Here we introduce Chroma, a generative model for proteins and protein complexes that can directly sample novel protein structures and sequences, and that can be conditioned to steer the generative process towards desired properties and functions. Given backbones from this diffusion process, the Chroma design network then generates sequence and side-chain conformations that are conditioned on the sampled backbone to yield a joint generative model for the sequences and structure of a protein complex. We sought to characterize the space of possible proteins parameterized by Chroma by generating a large number of unconditional samples of proteins and protein complexes (100,000 single-chain proteins and 20,000 complexes across two versions of the models, v.0 and v.1). The experimental characterization of 310 proteins shows that sampling from Chroma results in proteins that are highly expressed, fold and have favourable biophysical properties.

We reasoned that the best way to determine the plausibility of the protein space parameterized by Chroma was to draw independent samples from the model and test them experimentally. Our experimental validation shows that Chroma has learnt a sufficiently accurate distribution such that sampling from it results in proteins that express, fold, have favourable biophysical properties and conform to intended structures at non-trivial rates. The crystal structures of two designed proteins exhibit atomistic agreement with Chroma samples (a backbone root-mean-square deviation of around 1.0 Å). Moreover, the two designs with experimentally determined crystal structures demonstrate that a non-trivial fraction of this distribution should be expected to be atomistically accurate.

>MGSVEEVKRIMDLARQKISDAMDELNMDATLKQSVDESMKRAEQRAYELSKTHEKTDALGQASADLARELVARNTSEDHQKQIFEALKKAAEEMAHRSDSHEDRLVMALILQTYANAKVTFRILNSGKALGKEDEAQKMADRWTRLSAEAASLSVQAINDSTSAEKMAENFRQAKEDAVASLHRAGQDDLARKVSEFADAGLSKIDELMTLTGQMWAHGLFSKEWEDAARSLSRLAAVMLAQASQTKEGSLRAVKAMEKMADNAADEAEKLMKAGSENLYFQ[2x]>[2x]MKTISFNFNQFHQNEEQLKLQRDARISSNSVLELTKVVNGVPTWNSTGRALYAKPVQVWDSTTGNVASFETRFSFSIRQPFPRPH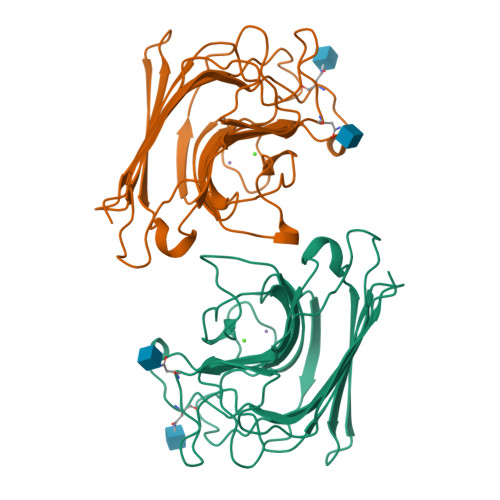PADGLVFFIAPPNTQTGEGGGYFGIYNPLSPYPFVAVEFDTFRNTWDPQIPHIGIDVNSVISTKTVPFTLDNGGIANVVIKYDASTKILHVVLVFPSLGTIYTIADIVDLKQVLPESVNVGFSAATGDPSGKQRNATETHDILSWSFSASLPGTNEF> YVPIP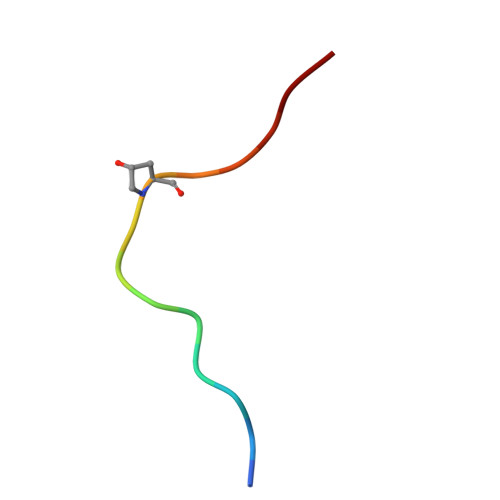PSAPSKRHN>ADPGKSCPSVCRCDAGFIYCNDRFLTSIPTGIPEDATTLYLQNNQINNAGIPSDLKNLLKVERIYLYHNSLDEFPTNLPKYVK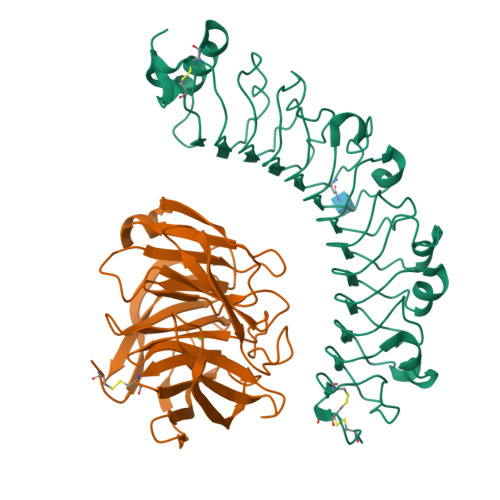ELHLQENNIRTITYDSLSKIPYLEELHLDDNSVSAVSIEEGAFRDSNYLRLLFLSRNHLSTIPWGLPRTIEELRLDDNRISTISSPSLQGLTSLKRLVLDGNLLNNHGLGDKVFFNLVNLTELSLVRNSLTAAPVNLPGTNLRKLYLQDNHINRVPPNAFSYLRQLYRLDMSNNNLSNLPQGIFDDLDNITQLILRNNPWYCGCKMKWVRDWLQSLPVKVNVRGLMCQAPEKVRGMAIKDLNAELFDCKD[4x];>[4x]VFLCPGLLKGVYQSEHLFESDHQSGAWCKDPLQASDKIYYMPWTPYRTDTLTEYSSKDDFIAGRPTTTYKLPHRVDGTGFVVYDGALFFNKERTRNIVKFDLRTRIKSGEAIIANANYHDTSPYRWGGKSDIDLAVDENGLWVIYATEQNNGKIVISQLNPYTLRIEGTWDTAYDKRSASNAFMICGILYVVKSVYEDDDNEATGNKIDYIYNTDQSKDSLVDVPFPNSYQYIAAVDYNPRDNLLYVWNNYHVVKYSLDFG>[3x]ATAAEIAALPRQKVELVDPPFVHAHSQVAEGGPKVVEFTMVIEEKKIVIDDAGTEVHAMAFNGTVPGPLMVVHQDDYLELTLINPETNTLMHN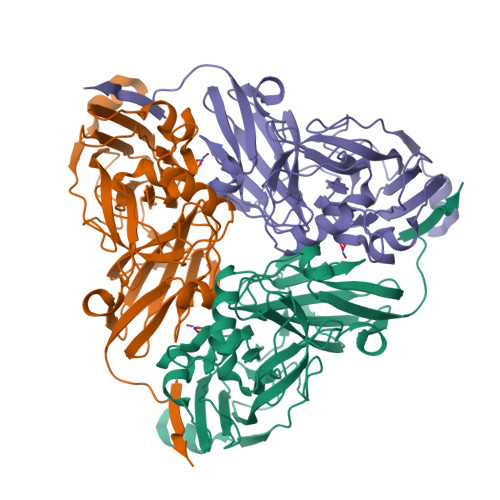IDFHAATGALGGGGLTEINPGEKTILRFKATKPGVFVYHCAPPGMVPWHVVSGMNGAIMVLPREGLHDGKGKALTYDKIYYVGEQDFYVPRDENGKYKKYEAPGDAYEDTVKVMRTLTPTHVVFNGAVGALTGDKAMTAAVGEKVLIVHSQANRDTRPHLGGGHGDYVWATGKFNTPPDVDQETWFIPGGAAGAAFYTFQQPGIYAYVNHNLIEAFELGAAAHFKVTGEWNDDLMTSVLAPSGTIEGR As for all other methanogenic pathways, the methyl group must be transferred onto coenzyme M (HS-CoM) to be released as methane by the Methyl-coenzyme M reductase (MCR). MCR is a three-subunit complex harboring the cofactor F430, a nickel-containing corrinoid that gives its yellow color to the enzyme. The chemical reaction catalyzed by the cofactor is a thiyl-radical mechanism in which the Ni(I)-active state will attack the thiol group of the methyl-S-CoM forcing the generation of methane and the formation of the heterodisulfide made of the HS-CoM and Coenzyme B (CoB-SH). In this report, we investigated MCR natively isolated from Methermicoccus shengliensis.

The structure of MCR from Methanosarcina barkeri (MbMCR) was used for molecular replacement based on a phylogenetic analysis and the MsMCR structure was refined to 1.6-Å resolution. The asymmetric unit contains two dimers with the typical (αβγ)2 organization. Interestingly, while the first dimer shows an excellent fit in the electron density (average B-factor = 22.6 Å2), the second dimer has a very high average B-factor (51.3 Å2), which made its accurate modelling challenging. The UV/Visible spectra is typical of the Ni(II) red1-silent state with an absorption peak at 424 nm. The active site is identical compared to the three other structural homologues with the same coordination of the coenzymes and F430-cofactor. Both coenzymes are bound at very high occupancy with a distance of 6.2 Å separating their sulphur groups as previously seen in other Ni(II) red1-silent structures, the density between the thiol groups was interpreted as a water molecule. The high quality of the obtained electron density map confirmed the presence of three modified residues: N1-methylhistidine275, 5(S)-methylarginine289, and the thioglycine463. Surprisingly, the S-methylcysteine and didehydroaspartate found in the close relatives M. barkeri and Methanosarcina acetivorans are not detected in M. shengliensis. Methanobacteriales, Methanococcales, Methanopyrus kandleri, and Methanoculleus thermophilus contain a 2(S)-methylglutamine close to the F430. This modification is not present in MbMCR and in M. acetivorans and the presented structural data shows a classic glutamine at this position in MsMCR. The electrostatic charge repartition of MsMCR fits very well with the one from MbMCR rather than the two other thermophiles showing that thermophilic and high salt adaptations of M. shengliensis have not drastically modified the enzyme surface.

>MTMVDREQLFKKALEIKFTQEWGENKATEVSTDITSKKAKYLRLGTAQSPRKREFEQYGKEIAAKRGLPGYDPKLHLGGIPLGQRQITPYVVSSTDTLCDGDDLHFVNNAAMQQMWDDIRRTVIVGMDLAHETLEKRLGKEVTPETINHYLEVLNHAMPGAAVVQEMMVETHPGLVDDCYVKVFTGDDELADEIDKRFLIDIDKQFGEEKAAQIKAAIGKTTWQAVHVPTIVVRTCDGATTSRWTAMQIGMSFIAAYRMCAGEAAVADLAYAAKHAALVGMGDMLPARRARGPNEPGGLQFGYLADIVQADRVTDDKVKASLEVVAAGAMLYDQIWLGSYMSGGVGFTQYATAAYTNNILDDFSYYGYEYAVDKYGGPAQAPATLETVKDIATETAIYAIEQYEYFPTLLEDQFGGSQRAAVVAAAAGIATGLATGNSQAGLSGWYLAQYLLKEAEGRLGFFGYDLQDQCGAANVFSYQSDEGLPLELRGPNYPNYAMNVGHQGEYAGIASSGHIGRGDAFVVNPLVKVAFADPLLNFDFTQVRKEFAKGAVREFDRCAGERALILPAK[4x];>MSDKVDIYSDRGKLLASDVDIMDLAPTRNRAIRTIIHDTKRTAAVNLGGIEKALANGRIGKVKKIPGKEMKLDIVANAERLAERVKELVQVNEGDDTTVEVLAGGKFLKVQVPSARLESGAEYVSSITASAAAITQAIIELFDVGIFDACMVKAAVWGDYPQTIGLNGGNVSSILEIPQKDEGLGFTLRNIMANHIAAITQRNAMNAAALSSILEQCGEFEMGNAIGMFERHQLLGLAYQGLNANNIVYETVKEQGKSGTIGTVVHSIVERALEDGVISVDKVAPSGYKFYKANDVMLWNAYAAAGSLAATMVNCGAARAAQCVSSTLLYFNDLLEKETGLPGCDYGKVQGTAVGFSFFSHSIYGGGGPGVFNGNHIVTRHSRGFAIPCVAAAVALDAGTQMFSPEMTSAVVGTVYGSIPEFREPIKTVAASL[4x];>[4x]MAYEPQYYPGNTSVAQNRRKHMSGNVEKLREISDEDLTAILGHRAPGSDYPSTHPPLAEMGEPDCPIREIVEPTPGAAAGDRIRYVQWTDSMYNAPATPYWRSYYAAINHRGVDPGTLSGRQIVEARERDVEVYGKMSIETEMTCPALAGLRGATVHGHSCRLQEDGVMFDMLDRRRLEGGTIIMDKDQVGVPLDRKVDLGKPMSEEEAAKRTTIYRVDNVPFRSDSEVVEWVQRIWELRTRYGFQPQ> EATECLTRSNLKKLQEKIFDRELNDIACDHCLCSTEN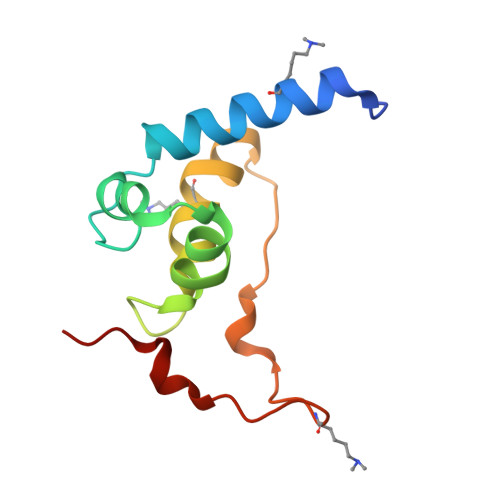RRDIKYSRLWFLFELEMSENWNENLRLSCYNKYVYSAIDESWKMENILLKEQEKHYEYFPIGQLLIPN> MSTNCFSGYKDLIKEGDLTLIWVSRDNIKPVRMHSEEVFNTRYGSFPHKDIIGKPYGSQIAIRTKGSNKFAFVHVLQPTPELWTLSLPHRTQIVYTPDSSYIMQRLNCSPHSRVIEAGTGSGSFSHAFARSVGHLFSFEFHHIRYEQALEEFKEHGLIDDNVTITHRDVCQGGFLIKKGDTTSYEFGNNETAASLNANVVFLDLPAPWDAIPHLDSVISVDEKVGLCCFSPCIEQVDKTLDVLEKYGWTDVEMVEIQGRQYESRRQMVRSLNDALERLRDIKRHKLQGVERRKRMFNNTIDSNDEKVGKRNEDGVPLTEKAKFNPFGKGSRIKEGDSNYKWKEVTKMEAEIKSH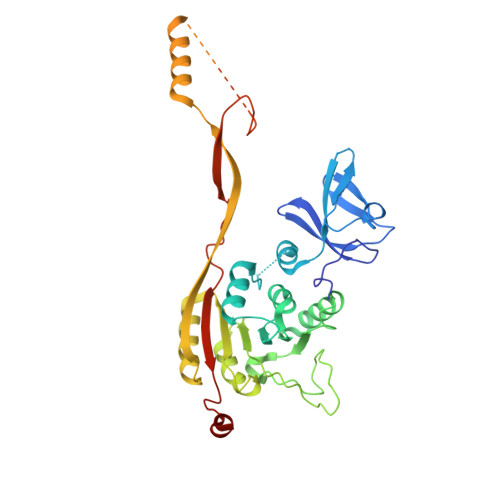TSYLTFAFKVVNRSRDDEKVNEILRSTEK>MKSSHHHHHHENLYFQSNAETIEIIKDLFEHLCGVRVHRTYEDDTGLWFDTSQGSKNGIMDYKLGFVKSQAENTTEVDTEVIYVPLLKQRTAEELQELQKKLPDYLFETLSFPLRSLNQFYIKMSKSLNKKV[4x];>[4x]DLKFKRHKNKHIQGFPTLGERLDNLQDIKKAKRVENFNSS

In S. cerevisiae meiosis I, sister kinetochores are fused through the action of the kinetochore-binding monopolin complex, and together bind a single microtubule. The conserved core of the monopolin complex comprises two nucleolar proteins, Csm1 and Lrs4. These proteins form a distinctive V-shaped complex, with two Csm1 homodimers bridged at their coiled-coil N-termini by a pair of Lrs4 subunits, thereby positioning two pairs of Csm1 globular-domain “heads” ~ 10 nm apart at the apices of the V. Each Csm1 globular domain has a conserved hydrophobic cavity implicated in binding the kinetochore protein Dsn1, leading to the proposal that monopolin could bridge Dsn1 molecules from sister kinetochores to physically fuse the kinetochores. A ~ 40-residue region within the disordered N-terminus of the core kinetochore protein, Dsn1, has been identified as the kinetochore receptor for the monopolin subunit Csm1.

The Cg Dsn1 Box 1-2-3 region shows high homology with the equivalent region of Sc Dsn1 (56% identity and 82% similarity between Sc Dsn1 residues 72–110 and Cg Dsn1 residues 32–67), and we were also able to reconstitute a complex of Cg Csm169–181 (56% identical to Sc Csm1 in this region) with Sc Dsn171–110. We crystallised and determined the structure of this chimeric complex to 2.5 Å resolution. In the crystal structures of both Cg Csm169–181:Dsn114–72 and the chimeric Cg Csm169–181:Sc Dsn171–110 complex, the Dsn1 Box 2–3 region wraps around the Csm1 globular domain, with Box 2 forming an α-helix that packs against the “side” of the Csm1 dimer, and Box 3 binding the Csm1 hydrophobic cavity. Box 2 is highly conserved in yeast with point centromeres, with an alternating pattern of hydrophobic (Sc Dsn1 L88/L92/L95) and polar (Sc Dsn1 E90/N94/D97) residues. In both structures, this region forms an α-helix oriented with the hydrophobic residues facing outward into solution, and the polar residues packed tightly against Csm1. This binding mode is unexpected, as hydrophobic residues are most often buried in protein-protein interfaces, rather than solvent-exposed. The core of the interaction comprises two conserved hydrophobic residues (Sc Dsn1 V104 and F107) inserted into the conserved hydrophobic cavity on Csm1. These residues are bracketed by positively charged amino acids (Sc Dsn1 K102 and R103) on the N-terminal side, and highly conserved serine residues (Sc Dsn1 S109 and S110) on the C-terminal side. Dsn1 Box 3 contains two serine residues (Sc Dsn1 S109 and S110) that are highly conserved throughout budding yeast. These serine residues are disordered in both crystal structures but are positioned close to conserved lysine residues in Csm1 (Cg Csm1 K172, K175, and K179).> MLPKRRRARVGSPSGDAASSTPPSTRFPGVAIYLVEPRMGRSRRAFLTGLARSKGFRVLDACSSEATHVVMEETSAEEAVSWQERRMAAAPPGCTPPALLDISWLTESLGAGQPVPVECRHRLEVAGPRKGPLSPAWMPAYACQRPTPLTHHNTGLSEALEILAEAAGFEGSEGRLLTFCRAASVLKALPSPVTTLSQLQGLPHFGEHSSRVVQELLEHGVCEEVERVRRSERYQTMKLFTQIFGVGVKTADRWYREGLRTLDDLREQPQKLTQQQKAGLQHHQDLSTPVLRSDVDALQQVVEEAVGQALPGATVTLTGGFRRGKLQGHDVDFLITHPKEGQEAGLLPRVMCRLQDQGLILYHQHQHSCCESPTRLAQQSHMDAFERSFCIFRLPQPGSWKAVRVDLVVAPVSQFPFALLGWTGSKLFARELRRFSRKEKGLWLNSHGLFDPEQKTFFQAASEEDIFRHLGLEYLPPEQRNA

Pol μ is capable of performing gap-filling repair synthesis in the nonhomologous end joining (NHEJ) pathway. Compared with replicative DNA polymerase, Pol μ lacks proofreading activity, with an intrinsically high error rate of 10−3–10−5 for dNTP incorporation. Here, crystal structures and kinetics of Pol μ substituting dGTP for dATP on gapped DNA substrates containing templating T were determined and compared.

To further investigate the possible roles of these two residues in dGTP misincorporation, crystal structures of Q441A single-mutant and Q441A/K438A double-mutant proteins complexed with 1-nt gapped DNA and dGMPNPP were determined (Complexes 4 and 5, respectively). In contrast to the stable templating T observed in all the WT:DNA structures (binary complex and Complexes 1-3), the electron density clearly shows an alternative conformation of the templating T and −1 base in the structure of Complex 4. The second conformation of templating T rolls toward the major groove but maintains its interactions with surrounding Arg residues. On the other side, the dGMPNPP and 3ʹ-end dA of the primer strand adopt a single conformation, which is very similar to the flipped conformation (conformation B) observed in Complexes 2 and 3. The N7 of guanine base of dGMPNPP interacts with Lys438, which forms a distorted WC-like pair with the templating T. Compared with WT:DNA structures (Complexes 2 and 3), structures in which alanine was substituted for Gln441 (Complexes 4 and 5) exhibit a much more stable dGMPNPP, indicating that Gln441 may play a role in discrimination against dGTP misincorporation over the templating T on a 1-nt gapped DNA substrate. This result is consistent with the increased Km for the correct insertion of dATP but a decreased Km for dGTP misincorporation of Q441A single-mutant and K438A/Q441A double-mutant proteins. In contrast, dGMPNPP is stable when Gln441 is replaced with Ala, leading to the destabilized templating strand (Complexes 4 and 5). Given that Q411A vs. WT exhibited both increased dGTP binding affinity and the elevated relative misincorporation rate on a 1-nt gapped DNA, Gln441 may function as the fidelity checkpoint in the minor groove by stabilizing the templating base.N-[(2R,4S,5S,7R)-4-AMINO-8-(BUTYLAMINO)-5-HYDROXY-2,7-DIMETHYL-8-OXOOCTYL]-2-(3-METHOXYPROPOXY)BENZAMIDE 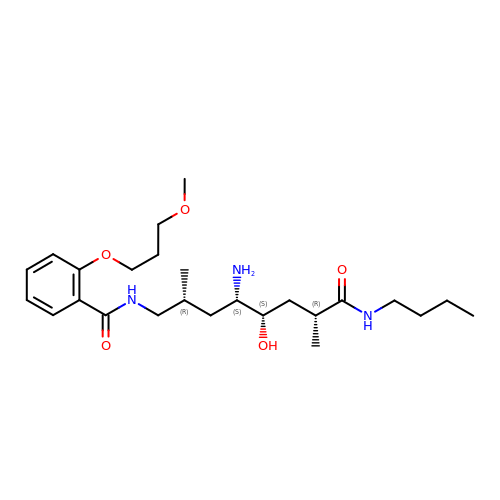| C25 H43 N3 O5 | HCEVFKSMFFEYMG-WKDRNLAYSA-N>[3x]MENKGEKIAMNPTVQTLAQKGDKLAVKLVTRGWASLSTNQKRRAEMLAGYTPAILAFTPRRPRMTNPPPRTSRNSPGQAGKSMTMSKTELLSTVKGTTGVIPSFEDWVVSPRNVAVFPQLSLLATNFNKYRITALTVKYSPACSFETNGRVALGFNDDASDTPPTTKVGFYDLGKHVETAAQTAKDLVIPVDGKTRFIRDSASDDAKLVDFGRIVLSTYGFDKADTVVGELFIQYTIVLSDPTKT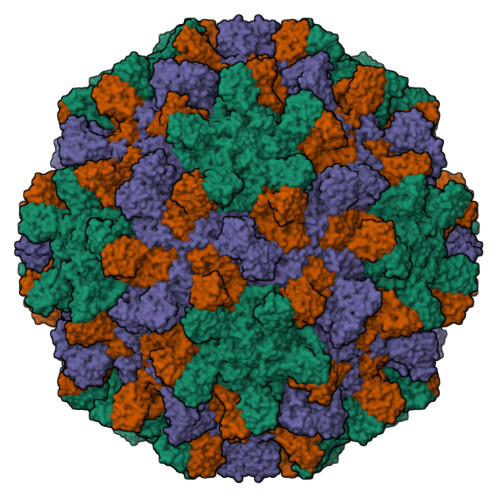AKISQASNDKVSDGPTYVVPSVNGNELQLRVVAAGKWCIIVRGTVEGGFTKPTLIGPGISGDVDYESARPIAVCELVTQMEGQILKITKTSAEQPLQWVVYRM>[4x]MGHHHHHHMVLADLGRKITSALRSLSNATIINEE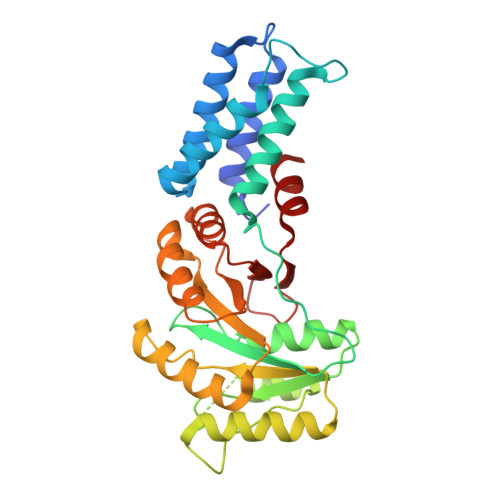VLNAMLKEVCTALLEADVNIKLVKQLRENVKSAIDLEEMASGLNKRKMIQHAVFKELVKLVDPGVKAWTPTKGKQNVIMFVGLQGSGKTTCSKLAYYYQRKGWKTCLICADTFRAGAFDQLKQNATKARIPFYGSYTEMDPVIIASEGVEKFKNENFEIIIVDTSGRHKQEDSLFEEMLQVANAIQPDNIVYVMDASIGQACEAQAKAFKDKVDVASVIVTKLDGHAKGGGALSAVAATKSPIIFIGTGEHIDDFEPFKTQPFISKLLG In mammals, fatty acid synthase (FASN) contains multiple enzymatic domains to catalyse all chemical reactions needed for de novo fatty acid synthesis. An ACP carries substrates from one enzyme to another, sequentially following the chemical reactions. In metazoans, all essential enzymes are included in a single polypeptide chain and are arranged into two main functional domains, each carrying out a key chemical process and named correspondingly the condensing and modifying domains. The entire cycle of fatty acid synthesis requires that ACP carries the substrate from one enzyme to another repeatedly. Here, using a strategy of tagging and purifying endogenous FASN in HEK293T cells for single-particle cryo-electron microscopy studies, we characterized the structural dynamics of endogenous human FASN.

During the condensing cycle, ACP shuttles its substrates between MAT and KS via a Ppant that is covalently linked to S2156. To capture intermediate conformations of ACP engaged with either KS or MAT, we combined particles of ACP-containing subsets from all three datasets to produce a single consensus composite map and subjected each wing to symmetry expansion followed by focused classification. This analysis produced 11 meaningful classes, which we grouped into 5 functional groups—ACP engaged with KS; ACP engaged with MAT; ACP between KS and MAT; and two different groups with ACP not seen. In the group of ACP engaged with KS (ACP–KS), an ACP density is captured in two positions attached to KS, revealing different levels of engagement. In one position (the grey density), a clear helical density is resolved in ACP interacting with H68 and K70 on the KS domain next to the catalytic cavity. We modelled this density as a Ppant arm attached to S2156. Visualizing Ppant density engaging with the KS catalytic site suggests that this is indeed a relevant snapshot of FASN in the condensing cycle. Mass spectrometry analysis confirms that purified FASN is full length with major post-translation modifications including Ppant modification on S2156, ensuring that FASN contains holo-ACP. Taking two substates, ACP–KS/dynamic MAT and ACP–MAT/dynamic MAT, as examples, the hot area of the ACP–KS/dynamic MAT substate extends from −20° to +60°, whereas that of the ACP–MAT/dynamic MAT substate is confined within −20° to +20°. This difference can be explained by the fact that KS is located closer to the linker and that the catalytic sites of KS and MAT face opposite sides of the condensing domain.

>[2x]MEEVVIAGMSGKLPESENLQEFWDNLIGGVDMVTDDDRRWKAGLYGLPRRSGKLKDLSRFDASFFGVHPKQAHTMDPQLRLLLEVTYEAIVDGGINPDSLRGTHTGVWVGVSGSETSEALSRDPETLVGYSMVGCQRAMMANRLSFFFDFRGPSIALDTACSSSLMALQNAYQAIHSGQCPAAIVGGINVLLKPNTSVQFLRLGMLSPEGTCKAFDTAGNGYCRSEGVVAVLLTKKSLARRVYATILNAGTNTDGFKEQGVTFPSGDIQEQLIRSLYQSAGVAPESFEYIEAHGTGTKVGDPQELNGITRALCATRQEPLLIGSTKSNMGHPEPASGLAALAKVLLSLEHGLWAPNLHFHSPNPEIPALLDGRLQVVDQPLPVRGGNVGINSFGFGGSNVHIILRPNTQPPPAPAPHATLPRLLRASGRTPEAVQKLLEQGLRHSQDLAFLSMLNDIAAVPATAMPFRGYAVLGGERGGPEVQQVPAGERPLWFICSGMGTQWRGMGLSLMRLDRFRDSILRSDEAVKPFGLKVSQLLLSTDESTFDDIVHSFVSLTAIQIGLIDLLSCMGLRPDGIVGHSLGEVACGYADGCLSQEEAVLAAYWRGQCIKEAHLPPGAMAAVGLSWEECKQRCPPGVVPACHNSKDTVTISGPQAPVFEFVEQLRKEGVFAKEVRTGGMAFHSYFMEAIAPPLLQELKKVIREPKPRSARWLSTSIPEAQWHSSLARTSSAEYNVNNLVSPVLFQEALWHVPEHAVVLEIAPHALLQAVLKRGLKPSCTIIPLMKKDHRDNLEFFLAGIGRLHLSGIDANPNALFPPVEFPAPRGTPLISPLIKWDHSLAWDVPAAEDFPNGS;> DXLMSVEVRQTLEREL> VCDSGNKEYMGIEVYVEATLDEPLRQTTCESEIHKYGASVSNGGLNISVDLLNCFLNFHTVGVYTNRDTVYAKFASLDPWTTEPMNSMTHDDLVKLTEECIVDIYLKCEVDKTKDFMKTNDNRLKPRDFKTVPPSNVGSMIELQSDYCVNDVTAYVKIYDECGNIKQHSIPTLRD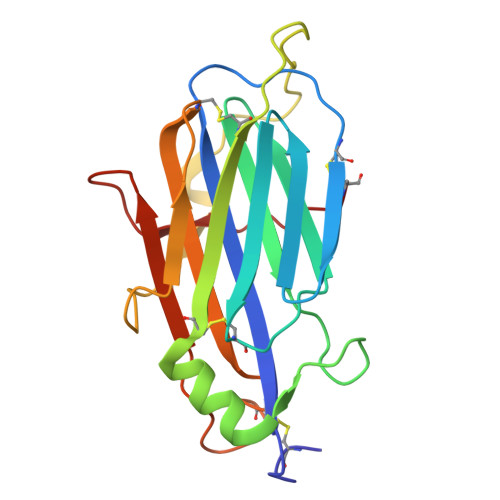YFTTKNGQPRKILKKKIDNC> VNRLDAIVWENIEGNLSRAFLTLDLHAFFNVNKEVGDGNCFYRALSRLHSESRTSNEHLYYRLLIPDAVDKYFDIEPEAIGLGLNKQEYVSKAILDGEWAGSLEASMLSKFLDITIIIWIVDDSGTIISANRYGEGRPSQAYNLCMVGNAHFDS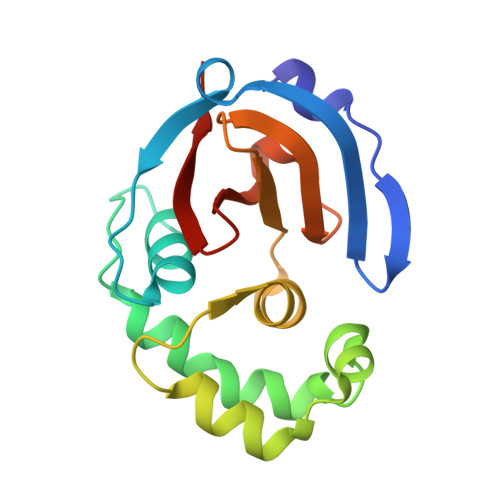LYIRV> GAAAGUGGGU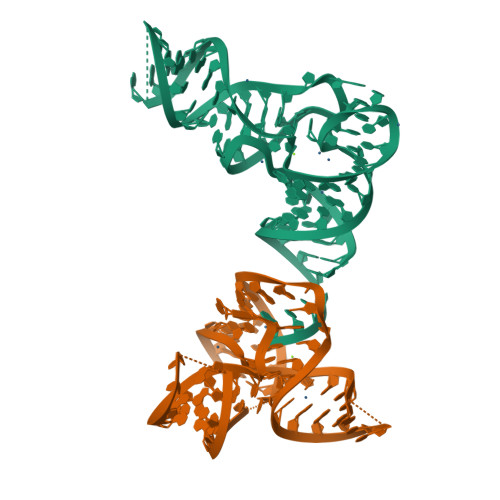GCGCGUUUGGCGCAUCAACUCGGGUGGAACCGCGGGAGCUACGCUCUCGUCCCGAG;> GCGGAAGUAGUUCAGUGGUAGAACACCACCUUGCCAAGGUGGGGGUCGCGGGUUCGAAUCCCGUCUUCCGCUCCA>MEITRLLTLYYEATPDPQNPLEGVRFGTSGHRGSSLKATFTEAHVLAIAQAIAELRPSFGATGPLFLAKDTHALSEPAWATALSVFAAHGIEVRVEADGDYTPTPLVSLAILEHNAHHEAKADGVLLTPSHNPPEDGGFKYNPPTGGPANARITRAIEERANALLQEGLKGVKRLPLREALARAKPFDYAGLYVEKVAEAVDLEAIRASGLRIGVDPLGGASLRVWERLAESHGLPLEVVNPTLDPTFRFMPKDHDGKIRMDCSSPYAMAGLLALKDRFDLAIGNDPDADRHGIVTPRGLMNPNHYLAAALHHLYTTRSWPGAKVGKTAVTSALLDRVAQALGREVYETPVGFKHFVAGLLEGWLGFAGEE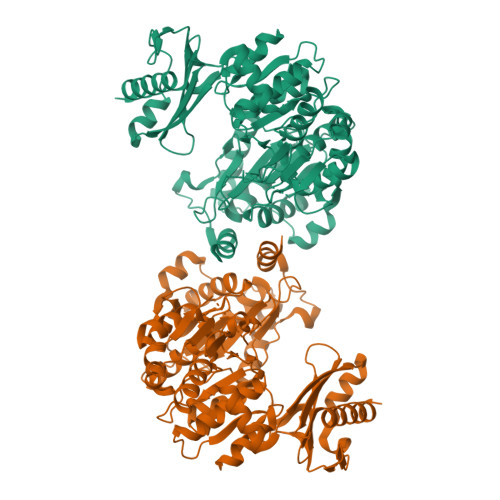SAGASFLRFDGRPFSTDKDGILMGLLAAELMAKRGQAPDALYEALAEKLGRPYYARKDLPVSPEAKARLARLSAKEVHPSTLAGEPVLQVLDRATGNGEPLGGIKVVAANAWFAVRPSGTEDVAKVYAESFLGEAHLERVLEEATALLHKALA[2x]>MKSSFSGKYQLQSQENFEAFMKAIGLPEELIQKGKDIKGVSEIVQNGKHFKFTITAGSKVI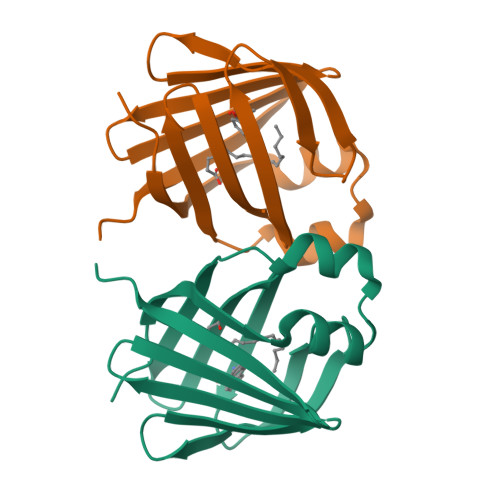QNEXTVGEEAEMETMTGEKVKTVVQLEGDNKLVTTFKNIKSVTELNGDIITNTMTLGDIVFKRISKRILEHHHHHH[2x]> DCSSGWSSYEGHCYKVFKQSKTWTDAES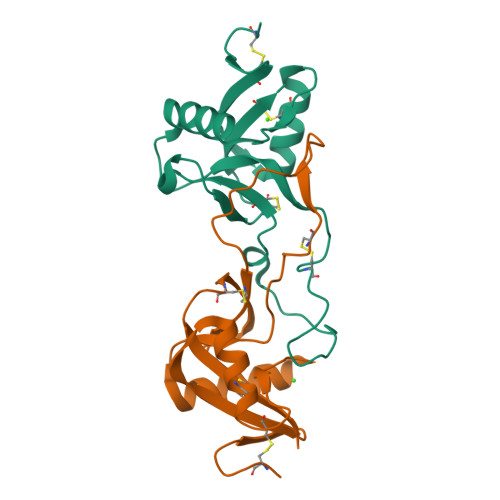FCTKQVNGGHLVSIESSGEADFVGQLIAQKIKSAKIHVWIGLRAQNKEKQCSIEWSDGSSISYENWIEEESKKCLGVHIETGFHKWENFYCEQQDPFVCEA;> DCPSDWSSYEGHCYKPFNEPKNWADAENFCTQQHTGSHLVSFQSTEEADFVVKLAFQTFDYGIFWMGLSKIWNQCNWQWSNAAMLKYTDWAEESYCVYFKSTNNKWRSITCRMIANFVCEFQA>GPHMKHPLMNVWTLWYLENDRSKSWEDMQNEITSFDTVEDFWSLYNHIKPPSEIKLGSDYSLFKKNIRPMWEDAANKQGGRWVITLNKSSKTDLDNLWLDVLLCLIG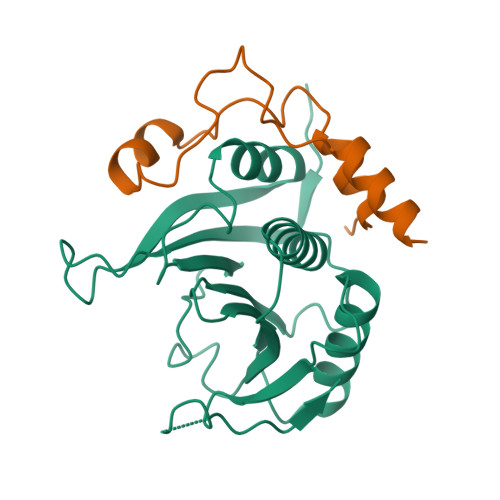EAFDHSDQICGAVINIRGKSNKISIWTADGNNEEAALEIGHKLRDALRLGRNNSLQYQLHKDTMVKQGSNVKSIYTL[4x];>[4x]GPHMLESRVSYDIEHLLYYSMSPHSWTLPTDWQKMQETAPSILRNKDLQDESQRFDGDKYLASIKTAAKR> MADVKLHGFWASPFSYRVIWALKLKGVEFEYIEEDLANKSELLLKYNPVYKQIPVFVHGGKPIAESLVILEYIEETWPENPLLPTDPYERAMARFWIQYGATKSAAFGALFRASGEELEKAAKEVVEVLRVLQEQGLGDKKFFGGDSINLVDISYGLFVYWLAAIEDIVGVKVLEPSTLPRLHAWAQNFIEVPLIKENHPDNDKLLL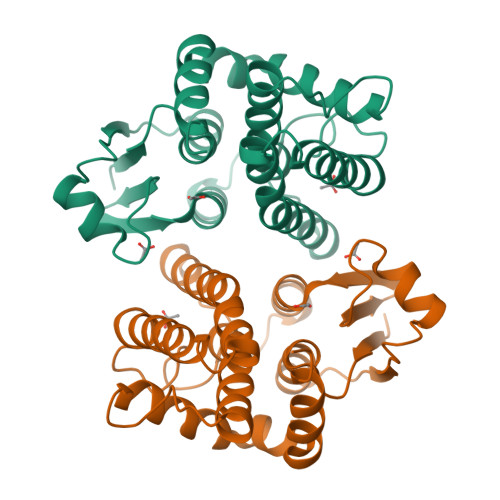HMKGVREKMMNK> MFENITAAPADPILGLADLFRADERPGKINLGIGVYKDETGKTPVLTSVKKAEQYLLENETTKNYLGIDGIPEFGRCTQELLFGKGSALINDKRARTAQTPGGTGALRVAADFLAKNTSVKRVWVSNPSWPNHKSVFNSAGLEVREYAYYDAENHTLDFDALINSLNEAQAGDVVLFHGCCHNPTGIDPTLEQWQTLAQLSVEKGWLPLFDFAYQGFARGLEEDAEGLRAFAAMHKELIVASSYSKNFGLYNERVGACTLVAADSETVDRAFSQMKAAIRANYSNPPAHGASVVATILSNDALRAIWEQELTDMRQRIQRMRQLFVNTLQEKGANR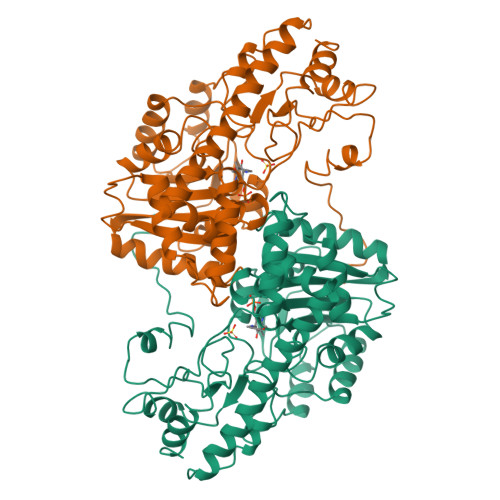DFSFIIKQNGMFSFSGLTKEQVLRLREEFGVYAVASGFVNVAGMTPDNMAPLCEAIVAVL>SQDASDGLQRLHMLQISYFRDPYHVWYQGNASLGGHLTHVLEGPDTNTTIIQLQPLQEPESWARTQSGLQSYLLQFHGLVRLVHQERTLAFPLTIRCFLGCELPPEGSRAHVFFEVAVNGSSFVSFRPERALWQADTQVTSGVVTFTLQQLNAYNRTRYELREFLEDTCVQYVQKHISAENTKGSQTSRSYTS[2x];>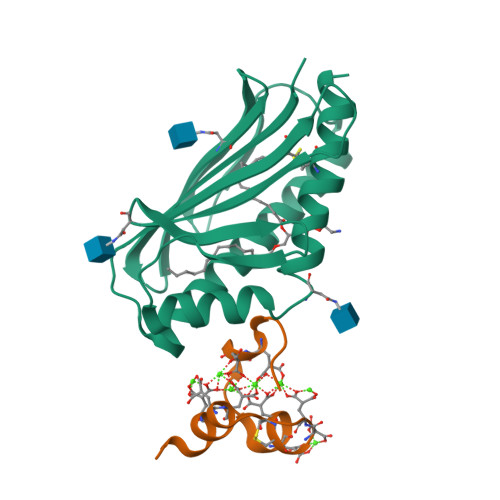ANSFLEELRHSSLERECIEEICDFEEAKEIFQN[2x]Protein splicing is catalyzed by intervening protein sequences termed inteins. The protein-splicing reaction involves the self-removal of the intein and concomitant joining of the two flanking sequences (exteins). All splicing domains found among inteins have the same structural architecture named HINT (Hedgehog/INTein) which relates to the C-terminal domain of the Hedgehog protein (Hh–C or hog domain). Instead of the N-terminal serine or cysteine missing among class 3 inteins, class 3 inteins contain an additional nucleophilic cysteine residue in block F.

We determined the high-resolution crystal structures of two variants of the class 3 MchDnaB1 intein (MchDnaB1_HN and MchDnaB1_HAA). As observed for other class 3 inteins, a mutation of the last Asn145 residue to Ala in the MchDnaB1 intein (MchDnaB1_HAA) largely halted the reaction at the branched acyl-intein intermediate. The WCT motif found in the class 3 intein participates in forming the catalytic triad, in which Cys124, His65, and Thr143 could serve as nucleophilic, basic, and acidic functional groups, respectively. Importantly, we could observe clear electron density near the side-chains of Cys124, His65, and the backbone of Val125 for both crystal structures of the MchDnaDB1_HN and MchDnaB1_HAA inteins (modeled as oxyanion waters in Figure 2a and Supplemental Figure S2). However, the crystal structures of both MchDnaB1 intein variants (HN and HAA at the C-terminus) lacked electron densities for the N-extein sequences. This observation is presumably due to self-cleavage at the N-terminus during sample preparation and/or crystallization (N-cleavage). On the other hand, the variant of MchDnaB1_HAA shows overall weaker densities for the second conformation in gauche+ for Cys124, which was not modeled. In the MchDnaB1_HAA intein bearing an extein residue, the distance between the Cβ atom of the +1 residue (Ala) and Sγ atom of Cys124 is 4.7–5.0 Å. However, this distance with the +1 residue of the C-extein would be much shorter (<3.0 Å) when the χ1 angle of Cys124 was in the trans conformation. The rotation of the χ1 angle of Cys124 could thus bring the nucleophilic atom sufficiently closer to the +1 residue, promoting the trans-esterification reaction step without requiring the substantial conformational changes reported for other class 1 intein structures.

>[2x]ALALYTPLPTPTGWTTMGDVAVGDELLGADGKPTRVVAATDVMLGRPCYEVEFSDGTVIVADAAHQWPTSGGIRTSAQLRSGADRIVVAGSAGGYAEQRSATGLLVPVVQIESARRVASVPVRCVEVDNPAHLYLAGRGMVPTHAA> MAVLKIISWNVNGLRAVHRKGFLKWFMEEKPDILCLQEIKAAPEQLPRKLRHVEGYRSFFTP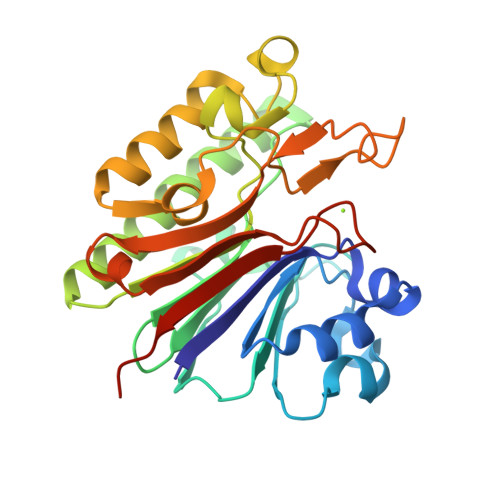AERKGYSGVAMYTKVPPSSLREGFGVERFDTEGRIQIADFDDFLLYNIYFPNGKMSEERLKYKLEFYDAFLEDVNRERDSGRNVIICGDFNTAHREIDLARPKENSNVSGFLPVERAWIDKFIENGYVDTFRMFNSDPGQYTWWSYRTRARERNVGWRLDYFFVNEEFKGKVKRSWILSDVMGSDHCPIGLEIELLEHHHHHH S-[2-({N-[(2R)-2-hydroxy-3,3-dimethyl-4-(phosphonooxy)butanoyl]-beta-alanyl}amino)ethyl] 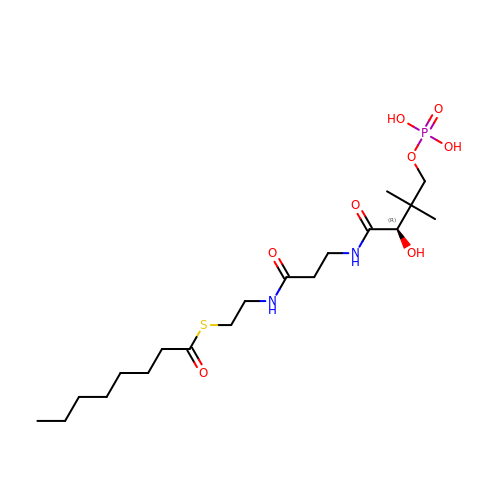octanethioate | C19 H37 N2 O8 P S | JIQRMRIKUIPMRV-KRWDZBQOSA-N>MVFAVDIIRHGDRTPIVALPTVNYQWQEGLGQLTAEGMQQEYKMGVAFRKKYIEELHLLPEHYEYGTIYVRSTDYARTLMSAQSLLMGLYPPGTGPSIPAGTSALPHAFQPIPVFSAPSKYDEVIIQQVDRKERKKLMEQYVFSTREWQQKNNELKDKYPLWSRLTGINIDTLEDLETVGHTLYVHQIHNAPMPEGLASNDIETIINSAEWAFMAQEKPQQIANVYSSKLMTNIADYLNSGSMKKSKLKYVLLSAHDTTIASVLSFLGAPLEKSPPYA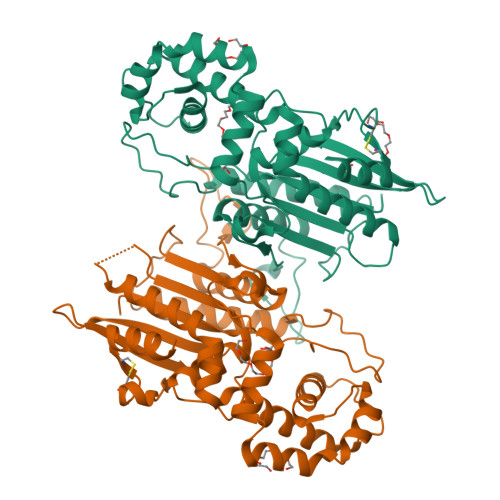SNVNFSLYDNGANYYTVKITYNGNPVLIPACGGSVCELQQLVNLVHDSKNLEHHHHHH[8x]> ADYDLKFGMNAGTSSNEYKAAEMFAKEVKEKSQGKIEISLYPSSQLGDDRAMLKQLKDGSLDFTFAESARFQLFYPEAAVFALPYVISNYNVAQKALFDTEFGKDLIKKMDKDLGVTLLSQAYNGTRQTTSNRAINSIADMKGLK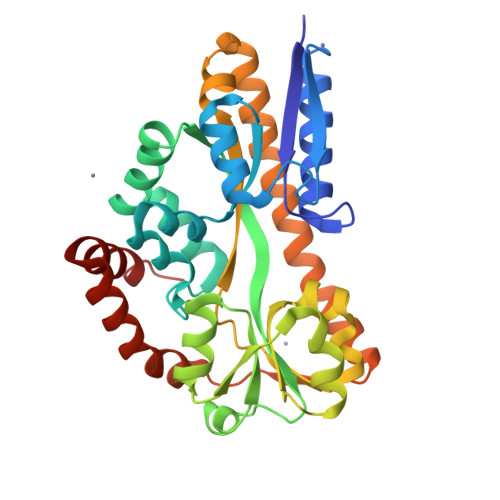LRVPNAATNLAYAKYVGASPTPMAFSEVYLALQTNAVDGQENPLAAVQAQKFYEVQKFLAMTNHILNDQLYLVSNETYKELPEDLQKVVKDAAENAAKYHTKLFVDGEKDLVTFFEKQGVKITHPDLVPFKESMKPYYAEFVKQTGQKGESALKQIEAINP>MARMNRPAPVEVTYKNMRFLITHNPTNATLNKFIEELKKYGVTTIVRVCEATYDTTLVEKEGIHVLDWPFDDGAPPSNQIVDDWLSLVKIKFREEPGCCIAVHSVAGLGRAPVLVA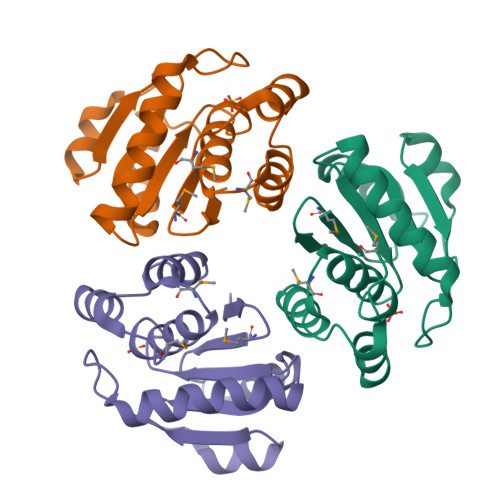LALIEGGMKYEDAVQFIRQKRRGAFNSKQLLYLEKYRPKMRLRFKDSNGHRNNCCIQ[6x]>[4x]FSPLSSQSSACCF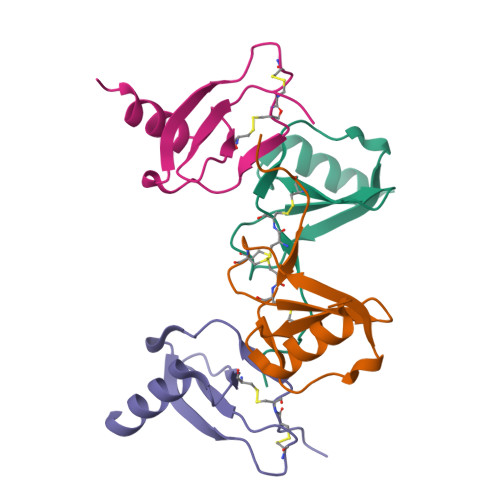AYIARPLPRAHIKEYFYTSGKCSNPAVVFVTRKNRQVCANPEKKWVREYINSLEMS> SAETQMERKIIDFLRQNGKSIALTIAKEIGLDKSTVNRHL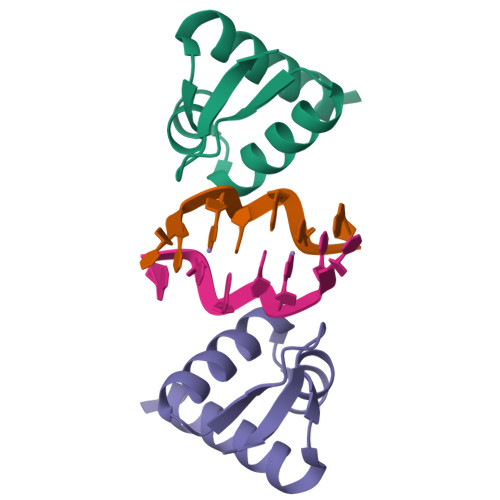YNLQRSNQVFNSNEKPPVWDLM> MASFSSYANGVKRWYQKLELPMPPERIFGAHMMLIGGLACLIGTYFFASMTMWNDGYVNLTLRPRLISLGIYDPYDTEQIQRVWLPLIGEFSTSKLPFFGQYPLTMTDFRLFGWGCFHIGLGLWLVYAGAAHYYGARGGATIGEIFWLLPYVPGLKGLCQIKWFTPEGPWYKVGLPWGSFANTPWPI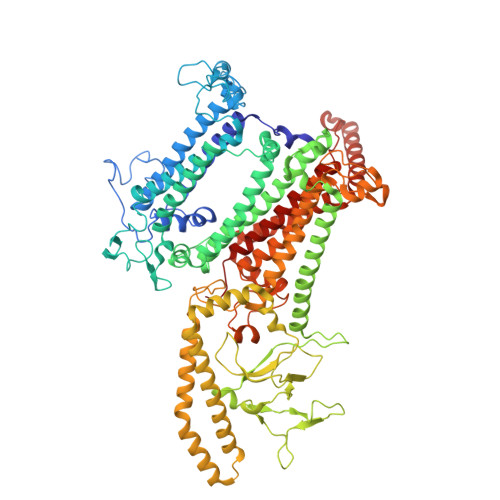LRRTYADALSPHTIYIGLLFFIWGFVLWFVLDKPPVPLQPAQVMTPNGLMPLEQAPFPYGWFDPYLNQVMHPMNTINGETTMCFVWGVLFVALGAYWWYRPPRSINITHLEDTKAVFHVHLTAIGYVSFALAIVGFLALRNHPSYLMLNDMNVIIYGKKIVNPGRMIHNMITFNHVQVGLLYVAAGVFHGGQYLHGLNISGAYKQARSKFITWFQNPDLQTKIVGTTMFVSFVTVVFGYGMICWNTGAELDLNFGIYQFRSFRAIQMDGEAGNIGYRVFRPKNPWDPTAGGDWVKNPDGTAKLVKARNLQVGDRILNEELGIGSSPTYSFTTIEEINYKPEWGQPKLYAVQWGSWTHFLRKVNPLFWVDKGIWYLQNQKTFEATRKADEAYLAAHLKAVSLLNQIDDAQTEEAKQKAQAELDKFRPELEKAHANMLEWNERLASTPAVLYSNLRDQHRDGEINDAIFFWLMIGGWLFGFIPLLRIAFHNYQSPWYRDFEWRKQSPDFPCIGPVKGGTCGVSIQDQLWFCILFSIKPLSAIAWYLDGGWIATMMARGNEAYYLTHNISHTGGVFLYMWNETTWIWTDNHLTAMLLLGHLIWFVSFALWFKDRGSRAEGGDIQSRWVRLMGKRLGIKTLQEVRFPVSNLATAKLWGTVFFYTGTFVLVFLYFADGFFQNR>[2x]GPGHMAQVAGAALSQAGWYLSDEGIEACTSSPDKVNVNDIILIALNTDLRTIGKKFLPSDINSGKVEKLEGPCVLQIQKIRNVAAPKDNEESQAAPRMLRLQMTDGHISCTAVEFSYMSKISLNTPPGTKVKLSGIVDIKNGFLLLNDSNTTVLGGEVEHLIEKW

Topoisomerase III (TOP3) is a member of the type IA topoisomerase family, which functions mainly in relaxing the supercoiled DNA and in resolving recombination intermediates during meiosis and DNA repair. TOP3β is an atypical topoisomerase that can recognize both DNA and RNA as the substrates12132223242526. Eukaryotic TOP3α and β are unique in that they interact with their specific auxiliary factors, RMI1 and TDRD3, respectively, and coexist with them in the cell. We determined the crystal structures of human TOP3β TOPO domain, TDRD3 DUF1767 and OB domains (DUF–OB) and their complex at 3.44 Å, 1.62 Å and 3.6 Å resolutions, respectively.

The N-terminal DUF1767 domain of TDRD3 is composed of four α-helices, followed by the β-barrel structure of the OB-fold domain. The DUF1767 structures of TDRD3 and RMI1 are topologically similar but differ in size and orientation relative to the OB-fold domain. The OB-fold domain of TDRD3 contains an insertion loop between β2 and β3 (Val79–Pro92), which is 23 residues shorter than that of RMI1 (Val95–Ser132). Concomitantly, the C-terminal region of the TDRD3 OB-fold domain is not folded into an α-helix, contrary to the secondary structure prediction by PSIPRED. Limited digestion with chymotrypsin cleaved the C-terminus of TDRD3 OB-fold at Trp161, which is positioned in the middle of the predicted α-helix. This result suggests that the C-terminal region of the TDRD3 OB-fold domain is unfolded in solution, consistent with the present structure. The insertion loop of TDRD3 is completely disordered in the apo TDRD3 and becomes ordered upon binding to TOP3β with some flexibility, as judged from high temperature factors. Comparison among the two apo TDRD3 structures in the asymmetric unit and the TOP3β-bound TDRD3 structure exhibited two different conformations around the N- and C-terminal ends of β3 and β4, respectively. β3 and β4 in one of the two apo TDRD3 molecules and the TOP3β-bound TDRD3 are one residue shorter than those in the other apo TDRD3 molecule. The Arg93-mediated hydrogen bonds stabilize the shorter β3 and β4, which might be appropriate for binding to TOP3β. We found a positively charged area that could be considered as the potential DNA/RNA-binding site in DUF–OB of TDRD3.> SNADAESLFREALSNKVDELAHFLLRKYRAKELVTKAEMLERVIKNYKRCFPVIFGKASESLKMIFGIDVKEVDPTSNTYTLVTCLGLSYDGLLGNNQIFPKTGLLIIVLGTIAMEGDSASEEE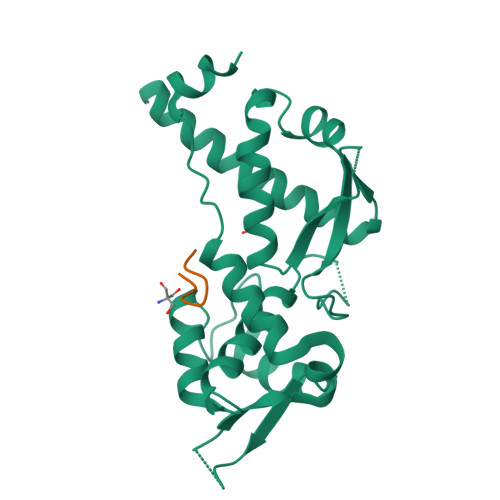IWEELGVMGVYDGREHTVYGEPRKLLTQDWVQENYLEYRQVPGSNPARYEFLWGPRALAETSYVKVLEHVVRVNARVRIAYPSLREAALLEEEEGV;> YIRLYDYHNC>MEFSVKSGSPEKQRSACIVVGVFEPRRLSPIAEQLDKISDGYISALLRRGELEGKPGQTLLLHHVPNVLSERILLIGCGKERELDERQYKQVIQKTINTLNDTGSMEAVCFLTELHVKGRNNYWKVRQAVETAKETLYSFDQLKTNKSEPRRPLRKMVFNVPTRRELTSGERAIQHGLAIAAGIKAAKDLGNMPPNICNAAYLASQARQLADSYSKNVITRVIGEQQMKELGMHSYLAVGQGSQNESLMSVIEYKGNASEDARPIVLVGKGLTFDSGGISIKPSEGMDEMKYDMCGAAAVYGVMRMVAELQLPINVIGVLAGCENMPGGRAYRPGDVLTTMSGQTVEVLNTDAEGRLVLCDVLTYVERFE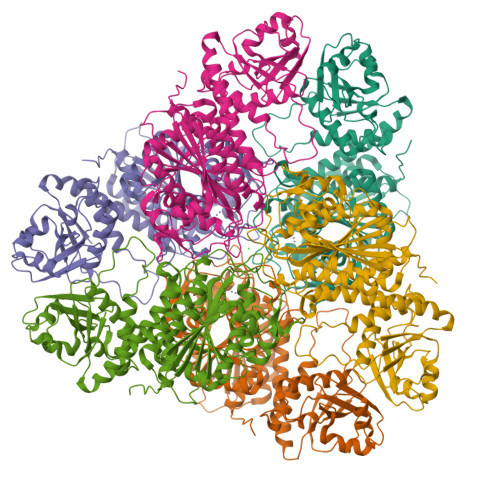PEAVIDVATLTGACVIALGHHITGLMANHNPLAHELIAASEQSGDRAWRLPLGDEYQEQLESNFADMANIGGRPGGAITAGCFLSRFTRKYNWAHLDIAGTAWRSGKAKGATGRPVALLAQFLLNRAGFNGEE[12x]>[14x]MSFDNYLVPT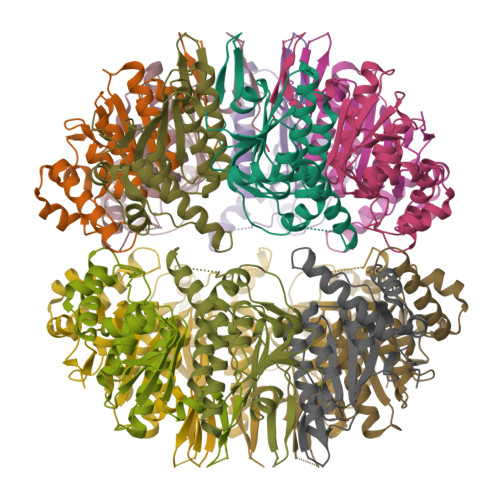VIEQSGRGERAFDIYSRLLKERIVFLVGPVTDESANLVVAQLLFLESENPDKDIFFYINSPGGSVTAGMSIYDTMNFIKPDVSTLCLGQAASMGAFLLSAGEKGKRFALPNSRIMIHQPLISGGLGGQASDIEIHARELLKIKEKLNRLMAKHCDRDLADLERDTDRDNFMSAEEAKEYGLIDQILENRASLQL>QGIREVILCKDQDGKIGLRLKSVDNGIFVQLVQANSPASLVGLRFGDQVLQINGENCAGWSSDKAHKVLKQAFGEKITMTIRDRPFERTVTMHKDSSGHVGFIFKSGKITSIVKDSSAARNGLLTDHHICEINGQNVIGLKDAQIADILSTAG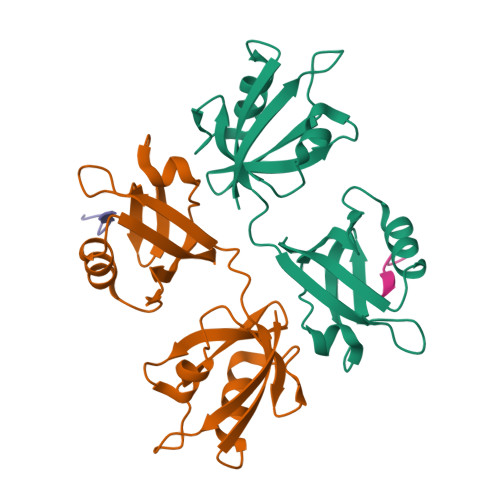TVVTITIMPA[4x];>[4x]APTNEFYA In Pectobacterium, iron acquisition via plant ferredoxin is mediated by the Ferredoxin uptake system (Fus), a molecular machine consisting of inner and outer membrane transporters and a periplasmically localised protease. Intriguingly, the outer membrane transporter from this system, a TonB-dependent transporter (TBDT) designated FusA, imports intact ferredoxin into the periplasm of the bacteria where it is processed by the M16 family protease FusC. To confirm the common architecture of these systems, we characterised the gene cluster analogous to the Fus from Escherichia coli: the ydd/pqqL operon. Furthermore, through structural and biochemical characterisation of the distantly related Fus homologues, YddB and PqqL from E. coli, we show that these proteins share key features with FusA and FusC, suggesting a conserved function.

We hypothesized that the uncharacterised protein PqqL, encoded in an operon with the yddB gene, is a protease that processes the substrate for this system upon import into the bacterial periplasm. PqqL consists of two clam-shell like halves, each formed from two M16 protease subunits.

>[2x]AALPQDEKLITGQLDNGLRYMIYPHAHPKDQVNLWLQIHTGSLQEEDNELGVAHFVEHMMFNGTKTWPGNKVIETFESMGLRFGRDVNAYTSYDETVYQVSLPTTQKQNLQQVMAIFSEWSNAATFEKLEVDAERGVITEEWRAHQDAKWRTSQARRPFLLANTRNLDREPIGLMDTVATVTPAQLRQFYQRWYQPNNMTFIVVGDIDSKEALALIKDNLSKLPANKAAENRVWPTKAENHLRFNIINDKENRVNGIALYYRLPMVQVNDEQSFIEQAEWSMLVQLFNQRLQERIQSGELKTISGGTARSVKIAPDYQSLFFRVNARDDNMQDAANALMAELATIDQHGFSAEELDDVKSTRLTWLKNAVDQQAERDLRMLTSRLASSSLNNTPFLSPEETYQLSKRLWQQITVQSLAEKWQQLRKNQDAFWEQMVNNEVAAKKALSPAAILALEKEYANKKLAAYVFPGR>MVTGGGAAPPGTVTEPLPSVIVLSAGRKMAAAAAAASGPGCSSAAGAGAAGVSEWLVLRDGCMHCDADGLHSLSYHPALNAILAVTSRGTIKVIDGTSGATLQASALSAKPGGQVKCQYISAVDKVIFVDDYAVGCRKDLNGILLLDTALQTPVSKQDDVVQLELPVTEAQQLLSACLEKVDISSTEGYDLFITQLKDGLKNTSHETAANHKVAKWATVTFHLPHHVLKSIASAIVNELKKINQNVAALPVASSVMDRLSYLLPSARPELGVGPGRSVDRSLMYSEANRRETFTSWPHVGYRWAQPDPMAQAGFYHQPASSGDDRAMCFTCSVCLVCWEPTDEPWSEHERHSPNCPFVKGEHTQNVPLSVTLATSPAQFPCTDGTDRISCFGSGSCPHFLAAATKRGKICIWDVSKLMKVHLKFEINAYDPAIVQQLILSGDPSSGVDSRRPTLAWLEDSSSCSDIPKLEGDSDDLLEDSDSEEHSRSDSVTGHTSQKEAMEVSLDITALSILQQPEKLQWEIVANVLEDTVKDLEELGANPCLTNSKSEKTKEKHQEQHNIPFPCLLAGGLLTYKSPATSPISSNSHRSLDGLSRTQGESISEQGSTDNESCTNSELNSPLVRRTLPVLLLYSIKESDEKAGKIFSQMNNIMSKSLHDDGFTVPQIIEMELDSQEQLLLQDPPVTYIQQFADAAANLTSPDSEKWNSVFPKPGTLVQCLRLPKFAEEENLCIDSITPCADGIHLLVGLRTCPVESLSAINQVEALNNLNKLNSALCNRRKGELESNLAVVNGANISVIQHESPADVQTPLIIQPEQRNVSGGYLVLYKMNYATRIVTLEEEPIKIQHIKDPQDTITSLILLPPDILDNREDDCEEPIEDMQLTSKNGFEREKTSDISTLGHLVITTQGGYVKILDLSNFEILAKVEPPKKEGTEEQDTFVSVIYCSGTDRLCACTKGGELHFLQIGGTCDDIDEADILVDGSLSKGIEPSSEGSKPLSNPSSPGISGVDLLVDQPFTLEILTSLVELTRFETLTPRFSATVPPCWVEVQQEQQQRRHPQHLHQQHHGDAAQHTRTWKLQTDSNSWDEHVFELVLPKACMVGHVDFKFVLNSNITNIPQIQVTLLKNKAPGLGKVNALNIEVEQNGKPSLVDLNEEMQHMDVEESQCLRLCPFLEDHKEDILCGPVWLASGLDLSGHAGMLTLTSPKLVKGMAGGKYRSFLIHVKAVNERGTEEICNGGMRPVVRLPSLKHQSNKGYSLASLLAKVAAGKEKSSNVKNENTSGTRKSENLRGCDLLQEVSVTIRRFKK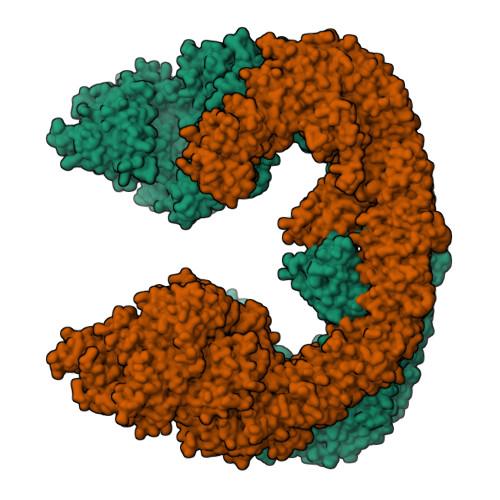TSISKERVQRCAMLQFSEFHEKLVNTLCRKTDDGQITEHAQSLVLDTLCWLAGVHSNGPGSSKEGNENLLSKTRKFLSDIVRVCFFEAGRSIAHKCARFLALCISNGKCDPCQPAFGPVLLKALLDNMSFLPAATTGGSVYWYFVLLNYVKDEDLAGCSTACASLLTAVSRQLQDRLTPMEALLQTRYGLYSSPFDPVLFDLEMSGSSCKNVYNSSIGVQSDEIDLSDVLSGNGKVSSCTAAEGSFTSLTGLLEVEPLHFTCVSTSDGTRIERDDAMSSFGVTPAVGGLSSGTVGEASTALSSAAQVALQSLSHAMASAEQQLQVLQEKQQQLLKLQQQKAKLEAKLHQTTAAAAAAASAVGPVHNSVPSNPVAAPGFFIHPSDVIPPTPKTTPLFMTPPLTPPNEAVSVVINAELAQLFPGSVIDPPAVNLAAHNKNSNKSRMNPLGSGLALAISHASHFLQPPPHQSIIIERMHSGARRFVTLDFGRPILLTDVLIPTCGDLASLSIDIWTLGEEVDGRRLVVATDISTHSLILHDLIPPPVCRFMKITVIGRYGSTNARAKIPLGFYYGHTYILPWESELKLMHDPLKGEGESANQPEIDQHLAMMVALQEDIQCRYNLACHRLETLLQSIDLPPLNSANNAQYFLRKPDKAVEEDSRVFSAYQDCIQLQLQLNLAHNAVQRLKVALGASRKMLSETSNPEDLIQTSSTEQLRTIIRYLLDTLLSLLHASNGHSVPAVLQSTFHAQACEELFKHLCISGTPKIRLHTGLLLVQLCGGERWWGQFLSNVLQELYNSEQLLIFPQDRVFMLLSCIGQRSLSNSGVLESLLNLLDNLLSPLQPQLPMHRRTEGVLDIPMISWVVMLVSRLLDYVATVEDEAAAAKKPLNGNQWSFINNNLHTQSLNRSSKGSSSLDRLYSRKIRKQLVHHKQQLNLLKAKQKALVEQMEKEKIQSNKGSSYKLLVEQAKLKQATSKHFKDLIRLRRTAEWSRSNLDTEVTTAKESPEIEPLPFTLAHERCISVVQKLVLFLLSMDFTCHADLLLFVCKVLARIANATRPTIHLCEIVNEPQLERLLLLLVGTDFNRGDISWGGAWAQYSLTCMLQDILAGELLAPVAAEAMEEGTVGDDVGATAGDSDDSLQQSSVQLLETIDEPLTHDITGAPPLSSLEKDKEIDLELLQDLMEVDIDPLDIDLEKDPLAAKVFKPISSTWYDYWGADYGTYNYNPYIGGLGIPVAKPPANTEKNGSQTVSVSVSQALDARLEVGLEQQAELMLKMMSTLEADSILQALTNTSPTLSQSPTGTDDSLLGGLQAANQTSQLIIQLSSVPMLNVCFNKLFSMLQVHHVQLESLLQLWLTLSLNSSSTGNKENGADIFLYNANRIPVISLNQASITSFLTVLAWYPNTLLRTWCLVLHSLTLMTNMQLNSGSSSAIGTQESTAHLLVSDPNLIHVLVKFLSGTSPHGTNQHSPQVGPTATQAMQEFLTRLQVHLSSTCPQIFSEFLLKLIHILSTERGAFQTGQGPLDAQVKLLEFTLEQNFEVVSVSTISAVIESVTFLVHHYITCSDKVMSRSGSDSSVGARACFGGLFANLIRPGDAKAVCGEMTRDQLMFDLLKLVNILVQLPLSGNREYSARVSVTTNTTDSVSDEEKVSGGKDGNGSSTSVQGSPAYVADLVLANQQIMSQILSALGLCNSSAMAMIIGASGLHLTKHENFHGGLDAISVGDGLFTILTTLSKKASTVHMMLQPILTYMACGYMGRQGSLATCQLSEPLLWFILRVLDTSDALKAFHDMGGVQLICNNMVTSTRAIVNTARSMVSTIMKFLDSGPNKAVDSTLKTRILASEPDNAEGIHNFAPLGTITSSSPTAQPAEVLLQATPPHRRARSAAWSYIFLPEEAWCDLTIHLPAAVLLKEIHIQPHLASLATCPSSVSVEVSADGVNMLPLSTPVVTSGLTYIKIQLVKAEVASAVCLRLHRPRDASTLGLSQIKLLGLTAFGTTSSATVNNPFLPSEDQVSKTSIGWLRLLHHCLTHISDLEGMMASAAAPTANLLQTCAALLMSPYCGMHSPNIEVVLVKIGLQSTRIGLKLIDILLRNCAASGSDPTDLNSPLLFGRLNGLSSDSTIDILYQLGTTQDPGTKDRIQALLKWVSDSARVAAMKRSGRMNYMCPNSSTVEYGLLMPSPSHLHCVAAILWHSYELLVEYDLPALLDQELFELLFNWSMSLPCNMVLKKAVDSLLCSMCHVHPNYFSLLMGWMGITPPPVQCHHRLSMTDDSKKQDLSSSLTDDSKNAQAPLALTESHLATLASSSQSPEAIKQLLDSGLPSLLVRSLASFCFSHISSSESIAQSIDISQDKLRRHHVPQQCNKMPITADLVAPILRFLTEVGNSHIMKDWLGGSEVNPLWTALLFLLCHSGSTSGSHNLGAQQTSARSASLSSAATTGLTTQQRTAIENATVAFFLQCISCHPNNQKLMAQVLCELFQTSPQRGNLPTSGNISGFIRRLFLQLMLEDEKVTMFLQSPCPLYKGRINATSHVIQHPMYGAGHKFRTLHLPVSTTLSDVLDRVSDTPSITAKLISEQKDDKEKKNHEEKEKVKAENGFQDNYSVVVASGLKSQSKRAVSATPPRPPSRRGRTIPDKIGSTSGAEAANKIITVPVFHLFHKLLAGQPLPAEMTLAQLLTLLYDRKLPQGYRSIDLTVKLGSRVITDPSLSKTDSYKRLHPEKDHGDLLASCPEDEALTPGDECMDGILDESLLETCPIQSPLQVFAGMGGLALIAERLPMLYPEVIQQVSAPVVTSTTQEKPKDSDQFEWVTIEQSGELVYEAPETVAAEPPPIKSAVQTMSPIPAHSLAAFGLFLRLPGYAEVLLKERKHAQCLLRLVLGVTDDGEGSHILQSPSANVLPTLPFHVLRSLFSTTPLTTDDGVLLRRMALEIGALHLILVCLSALSHHSPRVPNSSVNQTEPQVSSSHNPTSTEEQQLYWAKGTGFGTGSTASGWDVEQALTKQRLEEEHVTCLLQVLASYINPVSSAVNGEAQSSHETRGQNSNALPSVLLELLSQSCLIPAMSSYLRNDSVLDMARHVPLYRALLELLRAIASCAAMVPLLLPLSTENGEEEEEQSECQTSVGTLLAKMKTCVDTYTNRLRSKRENVKTGVKPDASDQEPEGLTLLVPDIQKTAEIVYAATTSLRQANQEKKLGEYSKKAAMKPKPLSVLKSLEEKYVAVMKKLQFDTFEMVSEDEDGKLGFKVNYHYMSQVKNANDANSAARARRLAQEAVTLSTSLPLSSSSSVFVRCDEERLDIMKVLITGPADTPYANGCFEFDVYFPQDYPSSPPLVNLETTGGHSVRFNPNLYNDGKVCLSILNTWHGRPEEKWNPQTSSFLQVLVSVQSLILVAEPYFNEPGYERSRGTPSGTQSSREYDGNIRQATVKWAMLEQIRNPSPCFKEVIHKHFYLKRVEIMAQCEEWIADIQQYSSDKRVGRTMSHHAAALKRHTAQLREELLKLPCPEGLDPDTDDAPEVCRATTGAEETLMHDQVKPSSSKELPSDFQLSAWSHPQFEK[2x]>[2x]MGHHHHHHSGMEQLSSANTRFALDLFLALSENNPAGNIFISPFSISSAMAMVFLGTRGNTAAQLSKTFHFNTVEEVHSRFQSLNADINKRGASYILKLANRLYGEKTYNFLPEFLVSTQKTYGADLASVDFQHASEDARKTINQWVKGQTEGKIPELLASGMVDNMTKLVLVNAIYFKGNWKD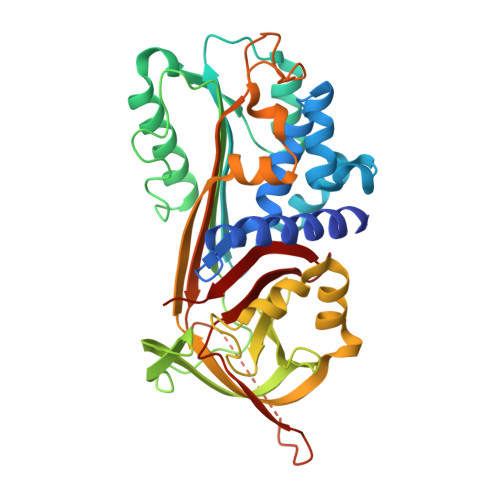KFMKEATTNAPFRLNKKDRKTVKMMYQKKKFAYGYIEDLKCRVLELPYQGEELSMVILLPDDIEDESTGLKKIEEQLTLEKLHEWTKPENLDFIEVNVSLPRFKLEESYTLNSDLARLGVQDLFNSSKADLSGMSGARDIFISKIVHKSFVEVNEEGTEAAAATAGIATFCMDDPEENFTADHPFLFFIRHNSSGSILFLGRFSSP>[2x]AAHLSDMLQQLHSVNASKPSERGLVRQEEAEDPACIPIFWVSKWVDYSDKYGLGYQLCDNSVGVLFNDSTRLILYNDGDSLQYIERDGTE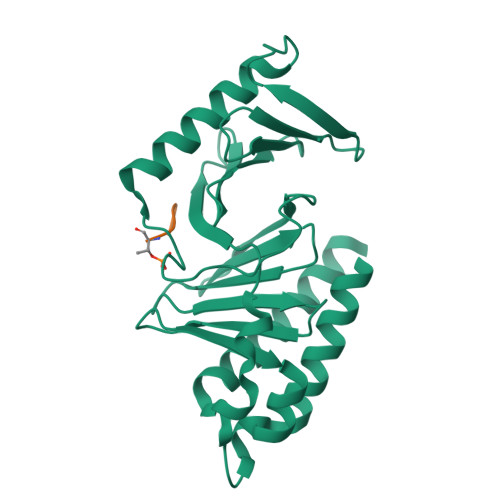SYLTVSSHPNSLMKKITLLKYFRNYMSEHLLKAGANITPREGDELARLPYLRTWFRTRSAIILHLSNGSVQINFFQDHTKLILCPLMAAVTYIDEKRDFRTYRLSLLEEYGCCKELASRLRYARTMVDKLLSSRSA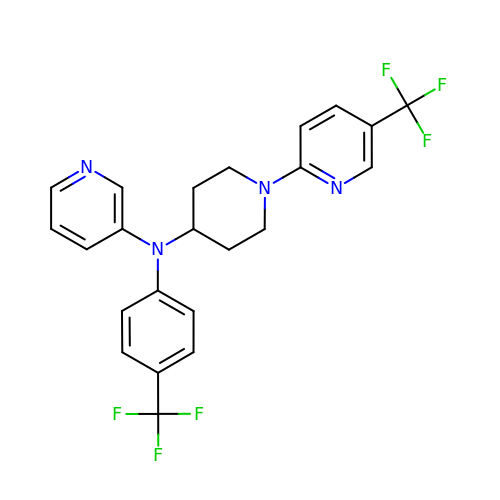N-[4-(trifluoromethyl)phenyl]-N-[1-[5-(trifluoromethyl)pyridin-2-yl]piperidin-4-yl]pyridin-3-amine | C23 H20 F6 N4 | XCJMUIWIEQFAQX-UHFFFAOYSA-N> MEYGHHARPDSKRPLDEGSPAAAGLTSKKANEALTRNRELTTVLVKNLPKSYNQNKVYKYFKHCGPIIHVDVADSLKKNFRFARIEFARYDGALAAITKTHKVVGQNEIIVSHLTECTLWMTNFPPSYTQRNIRDLLQDINVVALSIRLPSLRFNTSRRFAYIDVTSKEDARYCVEKLNGLKIEGYTLVTKVSNPLEKSKRTDSATLEGREIMIRNLSTELLDENLLRESFEGFGSIEKINIPAGQKEHSFNNCCAFMVFENKDSAERALQMNRSLLGNREISVSLADKKPFLERNEVK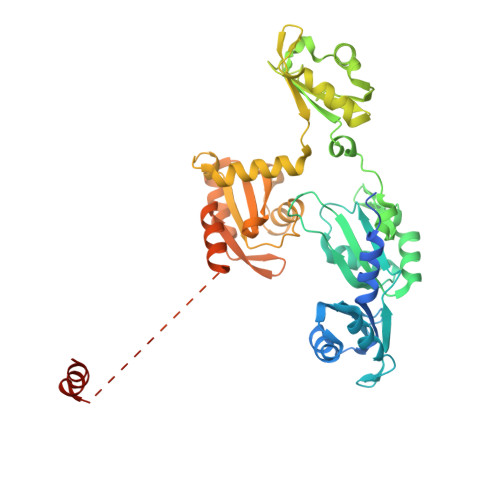RLLASRNSKELETLICLFPLSDKVSPSLICQFLQEEIHINEKDIRKILLVSDFNGAIIIFRDSKFAAKMLMILNGSQFQGKVIRSGTINDMKRYYNNQQNHSMKHVKPSCINMMEKGPNLQVKKKIPDKQEQMSNDDFRKMFLGELEHHHHHH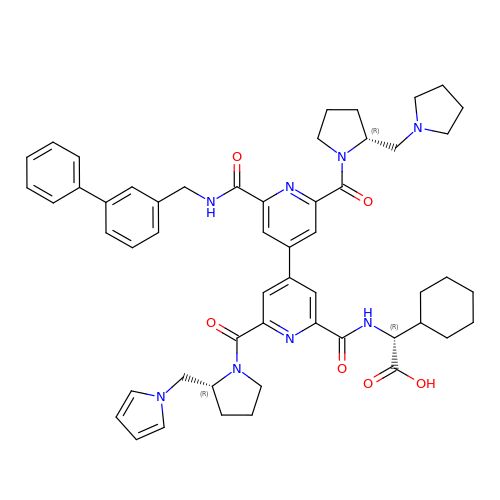(2R)-{[(2'-[(biphenyl-3-ylmethyl)carbamoyl]-6'-{[(2R)-2-(pyrrolidin-1-ylmethyl)pyrrolidin-1-yl]carbonyl}-6-{[(2R)-2-(1H-pyrrol-1-ylmethyl)pyrrolidin-1-yl]carbonyl}-4,4'-bipyridin-2-yl)carbonyl]amino}(cyclohexyl)ethanoic acid | C53 H60 N8 O6 | OURBCKKEKMWLAJ-JYIFATIISA-N(2S)-3-(7-carbamimidoylnaphthalen-2-yl)-2-[4-({(3R)-1-[(1Z)-ethanimidoyl]pyrrolidin-3-yl}oxy)phenyl]propanoic 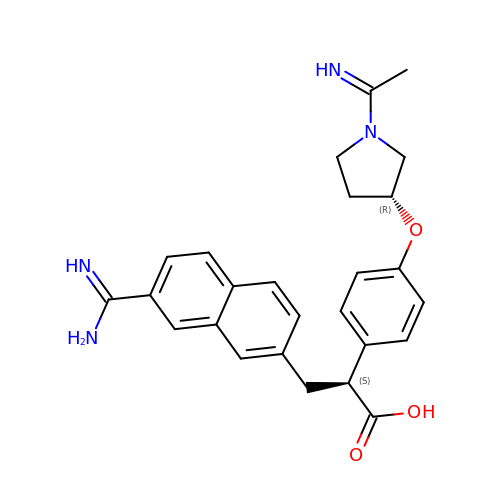acid | C26 H28 N4 O3 | AGRCGQSFFMCBRE-DGUCVARSSA-N>MDLHSLLELGTKPTAPHVRNKKVILFDTNHQVSICNQIIDAINSGIDLGDLLEGGLLTLCVEHYYNSDKDKFNTSPIAKYLRDAGYEFDVIKNADATRFLDVIPNEPHYSPLILALKTLESTESQRGRIGLFLSFCSLFLPKLVVGDRASIEKALRQVTVHQEQGIVTYPNHWLTTGHMKVIFGILRSSFILKFVLIYQGVNLVTGHDAYDSIISNSVGQTRFSGLLIVKTVLEFILQKTDSGVTLHPLVRTSKVKNEVASFKQALSNLARHGEYAPFARVLNLSGINNLEHGLYPQLSAIALGVATAHGSTLAGVNVGEQYQQLREAAYDAEVKLQRRHEHQEIQAIAEDDEERKILEQFHLQKTEITHSQTLAVLSQKREKLARLAAEIENNI[2x]

The nucleoprotein (NP) of Marburg virus (MARV), a close relative of Ebola virus (EBOV), encapsidates the single-stranded, negative-sense viral genomic RNA (vRNA) to form the helical NP–RNA complex. The NP–RNA complex constitutes the core structure for the assembly of the nucleocapsid that is responsible for viral RNA synthesis. Similar to EBOV NP, MARV NP possesses the structural domains: an N-terminal arm, an NP core composed of N- and C-terminal lobes, a disordered linker, and a C-terminal tail. The core structure of RNA-free monomeric MARV NP, spanning residues 21–373, features a typical bilobed fold consisting of N-terminal and C-terminal lobes, as determined using X-ray crystallography at 2.9 Å resolution, which is similar to that of the EBOV NP core structure. These two lobes are connected by a flexible hinge region and are considered to clamp the RNA strand between the two lobes by electrostatic interactions.

Here, we show the structure of the MARV NP–RNA complex determined using cryo-electron microscopy at a resolution of 3.1 Å. The constituted complex shows a left-handed double-helical structure, in which respective strands have similar dimensions: each strand contains single-strand RNA, and 30.50 NP subunits per turn and a 128.99 Å helical pitch (rise = 4.23 Å, rotation = 11.8052°) with the outer and inner diameters of ~330 Å and 255 Å, respectively. In the cryo-EM map, the density of the nucleotide bases and most of the side chains are clearly visible, which enabled us to build an atomic model unambiguously showing six RNA nucleotides enclosed by the N- and C-terminal lobes of NP. The respective asymmetric NP subunits, NP-a and NP-b, show very similar conformations as shown by a 0.592 Å backbone Root Mean Square Deviation (RMSD). In the positively charged cleft between the N- and C-terminal lobes, six RNA nucleotides are encapsidated with a “3-bases-inward, 3-bases-outward” configuration. In particular, the interactions between NP and RNA are predominantly electrostatic due to positively charged residues such as K142, K153, R156, and H292 with their side chains pointing to the phosphate backbone of the RNA. The N-terminal arm (residues 1 to 19) protrudes sideway from the N-terminal lobe and has a short 310-helix η1, which is associated with a neighboring NP molecule within the helical complex. Similar to EBOV NP, the N-terminal arm of MARV NPn occupies a hydrophobic pocket located on the C-terminal lobe of NPn+1 via L6 and L9. In our model, helix α15 of NPn is associated with α16 of the adjacent NPn+1, which is mediated by hydrophobic interactions between a hydrophobic patch composed of L249, L325, and L336 on NPn and a hydrophobic region composed of I357, F361, and I368 on NPn+1. The structures of the asymmetric unit, a complex of an NP and six RNA nucleotides, was very similar to that of EBOV, suggesting that both viruses share common mechanisms for the nucleocapsid formation.>MASEVVCGLIFRLLLPICLAVACAFRYNGLSFVYLIYLLLIPLFSEPTKATMQGHTGRLLQSLCITSLSFLLLHIIFHITLASLEAQHRITPAYNCSTWEKTFRQIGFESLKGADAGNGIRVFVPDIGMFIASLTIWLVCRTIVKKPDTEEIAQLNSECENEELAGGEKMDSEEALIYEEDLDGEEGMEGELEESTKLKILRRFASVASKLKEFIGNMITTAGKVVVTILLGSSGMMLPSLTSAVYFFVFLGLCTWWSWCRTFDPLLFGCLCVLLAIFTAGHLIGLYLYQFQFFQEAVPPNDYYARLFGIKSVIQTDCASTWKIIVNPDLSWYHHANPILLLVMYYTLATLIRIWLQEPLVQEEMAKEDEGALDCSSNQNTAERRRSLWYATQYPTDERKLLSMTQDDYKPSDGLLVTVNGNPVDYHTIHPSLPIENGPAKTDLYTTPQYRWEPSEESSEKKEEEEDKREDSEGEGSQEEKRSVRMHAMVAVFQFIMKQSYICALIAMMAWSITYHSWLTFVLLIWSCTLWMIRNRRKYAMISSPFMVVYANLLLVLQYIWSFELPEIKKVPGFLEKKEPGELASKILFTITFWLLLRQHLTEQKALREKEALLSEVKIGSQELEEKEDEELQDVQVEGEPTEKEEEEEEEIKEERHEVKKEEEEEVEEDDDQDIMKVLGNLVVALFIKYWIYVCGGMFFFVSFEGKIVMYKIIYMVLFLFCVALYQVHYEWWRKILKYFWMSVVIYTMLVLIFIYTYQFENFPGLWQNMTGLKKEKLEDLGLKQFTVAELFTRIFIPTSFLLVCILHLHYFHDRFLELTDLKSIPSKEDNTIYSHAKVNGRVYLIINRLAHPEGSLPDLAIMNMTASLDKPEVQKLAESGEERPEECVKKTEKGEAGKDSDESEEEEDEEEESEEEESSDLRNKWHLVIDRLTVLFLKFLEYFHKLQVFMWWILELHIIKIVSSYIIWVTVKEVSLFNYVFLISWAFALPYAKLRRAASSVCTVWTCVIIVCKMLYQLQTIKPENFSVNCSLPNENQTNIPLHELNKSLLYSAPVDPTEWVGLRKSSPLLVYLRNNLLMLAILAFEVTVYRHQEYYRGRNNLTAPVSKTIFHDITRLHLDDGLINCAKYFVNYFFYKFGLETCFLMSVNVIGQRMDFYAMIHACWLIGVLYRRRRKAIAEVWPKYCCFLACIITFQYFVCIGIPPAPCRDYPWRFKGAYFNDNIIKWLYFPDFIVRPNPVFLVYDFMLLLCASLQRQIFEDENKAAVRIMAGDNVEICMNLDAASFSQHNPVPDFIHCRSYLDMSKVIIFSYLFWFVLTIIFITGTTRISIFCMGYLVACFYFLLFGGDLLLKPIKSILRYWDWLIAYNVFVITMKNILSIGACGYIGALVRNSCWLIQAFSLACTVKGYQMPEDDSRCKLPSGEAGIIWDSICFAFLLLQRRVFMSYYFLHVVADIKASQILASRGAELFQATIVKAVKARIEEEKKSMDQLKRQMDRIKARQQKYKKGKERMLSLTQESGEGQDIQKVSEEDDEREADKQKAKGKKKQWWRPWVDHASMVRSGDYYLFETDSEEEEEEELKKEDEEPPRKSAFQFVYQAWITDPKTALRQRRKEKKKLAREEQKERRKGSGDGPVEWEDREDEPVKKKSDGPDNIIKRIFNILKFTWVLFLATVDSFTTWLNSISREHIDISTVLRIERCMLTREIKKGNVPTRESIHMYYQNHIMNLSRESGLDTIDEHSGAGSRAQAAHRMDSLDSRDSISSCYTEATLLISRQSTLDDLDGQDPVPKTSERARPRLRKMFSLDMSSSSADSGSVASSEPTQCTMLYSRQGTTETIEEVEAEAEEEVVEGLEPELHDAEEKEYAAEYEAGVEEISLTPDEELPQFSTDDCEAPPSYSKAVSFEHLSFASQDDSGAKNHMVVSPDDSRTDKLESSILPPLTHELTASDLLMSKMFHDDELEESEKFYVDQPRFLLLFYAMYNTLVARSEMVCYFVIILNHMTSASIITLLLPILIFLWAMLSVPRPSRRFWMMAIVYTEVAIVVKYFFQFGFFPWNKDLEIYKERPYFPPNIIGVEKKEGYVLYDLIQLLALFFHRSILKCHGLWDEDDIVDSNTDKEGSDDELSLDQGRRGSSDSLKSINLAASVESVHVTFPEQPAAIRRKRSCSSSQISPRSSFSSNRSKRGSTSTRNSSQKGSSVLSLKQKSKRELYMEKLQEHLIKAKAFTIKKTLQIYVPIRQFFYDLIHPDYSAVTDVYVLMFLADTVDFIIIVFGFWAFGKHSAAADITSSLSEDQVPGPFLVMVLIQFGTMVVDRALYLRKTVLGKVIFQVILVFGIHFWMFFILPGVTERKFSQNLVAQLWYFVKCVYFGLSAYQIRCGYPTRVLGNFLTKSYNYVNLFLFQGFRLVPFLTELRAVMDWVWTDTTLSLSSWICVEDIYAHIFILKCWRESEKRYPQPRGQKKKKAVKYGMGGMIIVLLICIVWFPLLFMSLIKSVAGVINQPLDVSVTITLGGYQPIFTMSAQQSQLKVMDNSKYNEFLKSFGPNSGAMQFLENYEREDVTVAELEGNSNSLWTISPPSKQKMIQELTDPNSCFSVVFSWSIQRNMTLGAKAEIATDKLSFPLAVATRNSIAKMIAGNDTESSNTPVTIEKIYPYYVKAPSDSNSKPIKQLLSENNFMNITIILFRDNVTKSNSEWWVLNLTGSRIFNQGSQALELVVFNDKVSPPSLGFLAGYGIMGLYASVVLVIGKFVREFFSGISHSIMFE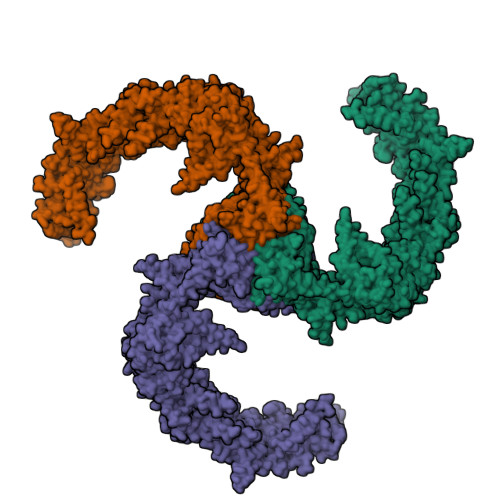ELPNVDRILKLCTDIFLVRETGELELEEDLYAKLIFLYRSPETMIKWTREKTN[3x]> GAMASELTPEERSELKNSIAEFHTYQLDPGSCSSLHAQRIHAPPELVWSIVRRFDKPQTYKHFIKSCSVE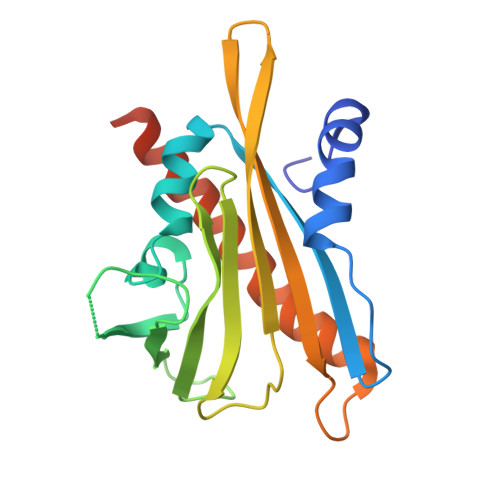QNFEMRVGCTRDVIVISGLPANTSTERLDILDDERRVTGFSIIGGEHRLTNYKSVTTVHRFEKENRIWTVVLESYVVDMPEGNSEDDTRMFADTVVKLNLQKLATVAEAMARNSGDGSGSQVT Like E1 enzymes, aminoacyl tRNA synthetases (aaRSs) are adenylate-forming enzymes (AFEs). They catalyze the transformation of amino acids into AMP conjugates, and then into aminoacyl-tRNAs, to supply protein synthesis. PfYRS is a Class I aaRS, characterized by a catalytic domain that adopts a Rossmann fold (residues 18–260) linked to a C-terminal domain (residues 261–370) that is involved in recognition of the anticodon stem of tRNATyr. PfYRS contains the two motifs characteristic of the catalytic domain of Class I (sub-class c) tRNA synthetases: “HIGH” and “KMSKS” (70HIAQ73 and 247KMSKS251 in PfYRS).

Whole genome sequencing of one parental and three resistant clones revealed nine newly acquired mutations in the resistant clones, three of which were in PF3D7_0807900 (position 403,556), corresponding to a Ser234Cys mutation in cytoplasmic PfYRS. YRSs from wildtype (PfYRS), mutant (PfYRSS234C) and human (mature HsYRS) were produced in Escherichia coli. Thus, it appears that the ability of PfYRS to catalyze formation of the ML901-Tyr conjugate is the primary factor controlling selectivity versus HsYRS and potency versus PfYRSS234C. That is, the decreased susceptibility of HsYRS and PfYRSS234C to reaction hijacking by ML901 is associated with mobility of the KMSSS/KMSKS loop, which is, in turn, associated with rotation of the His49/70 side chain. These conformational changes may promote dissociation of the charged tRNA, thereby preventing the hijacking reaction.

>[2x]GETTDTKREEQEIEEKKAQEESKIEDVDKILNDILSISSECIQPDELRVKLLLKRKLICYDGFEPSGRMHIAQGLLKSIIVNKLTSNGCTFIFWIADWFAHLNNKMSGDLKKIKKVGSYFIEVWKSCGMNMENVQFLWASEEINKKPNEYWSLVLDISRSFNINRMKRCLKIMGRSEGEENYCSQILYPCMQCADIFFLNVDICQLGIDQRKVNMLAREYCDIKKIKKKPVILCHGMLPGLLEGQEKMSKSDENSAIFMDDSESDVNRKIKKAYCPPNVIENNPIYAYAKSIIFPSYNEFNLVRKEKNGGDKTYYTLQELEHDYVNGFIHPLDLKDNVAMYINKLLQPVRDHFQNNIEAKNLLNEIKKYKVTK We characterized the evolutionary trajectories and selection forces underlying emergence of β-propeller proteins, a globular and symmetric fold group with diverse functions. Propellers comprise four to eight blades arranged in radial symmetry, with each blade comprising a four-strand β sheet. Second, tachylectin-2 is an immunoprotein that agglutinates foreign cells by multivalent binding of surface GlcNAc- and GalNAc-decorated glycoproteins. The repeating motifs encode both the globular propeller fold and the rigid binding of saccharides between propeller blades.

First, we show that single ancestral motifs inferred from the sequence repeats of the extant propeller yield a functional lectin via oligomerization. The best performing sequence from the first round of selection (Anc1B library) was subjected to error-prone PCR at a rate of 1.6 mutations per motif. Selection identified a single mutation, F23L (AncB1B), which was incidentally an ancestral state predicted with low probability; this mutant exhibited similar total binding capacity to AncA1B. AncA1B and AncB1B were purified with a sugar ligand (GlcNAc) resin and eluted indistinguishably from WT tachylectin-2 in gel filtration, indicating the formation of stable pentamers; additional peaks corresponding to alternate states were not observed. The crystal structure of AncB1B was essentially identical to the WT structure despite its alternate permutation frame, with each of the pentameric subunits cradling GlcNAc in the same binding orientation as the five-bladed WT monomer. The repetitively observed mutations of selected single motifs localized along the subunit interfaces and near the GlcNAc binding sites. The pentameric single motifs showed a bell-shaped curve of concentration-dependent folding efficiency, indicating that native pentamer formation was favored at higher concentrations but was simultaneously compromised by misfolding intermolecular interactions (blue lines). Single motifs unfolded in a simple two-state transition. A moderately stable oligomeric assembly enabled the emergence of functional single motifs.

>MSGFKFLFFSPDGTLYGVHNDKLYKGTPPTSDNDNWLARATLIGNGGW[15x]>MHNDKDLSTWQTFRRLWPTIAPFKAGLIVAGIALILNAASDTFMLSLLKPLLDDGFGKTDRSVLLWMPLVVIGLMILRGITSYISSYCISWVSGKVVMTMRRRLFGHMMGMPVAFFDKQSTGTLLSRITYDSEQVASSSSGALITVVREGASIIGLFIMMFYYSWQLSIILVVLAPIVSIAIRVVSKRFRSISKNMQNTMGQVTTSAEQMLKGHKEVLIFGGQEVETKRFDKVSNKMRLQGMKMVSASSISDPIIQLIASLALAFVLYAASFPSVMDSLTAGTITVVFSSMIALMRPLKSLTNVNAQFQRGMAACQTLFAILDSEQEKDEGKRVIDRATGDLEFRNVTFTYPGREVPALRNINLKIPAGKTVALVGRSGSGKSTIASLITRFYDIDEGHILMDGHDLREYTLASLRNQVALVSQNVHLFNDTVANNIAYARTEEYSREQIEEAARMAYAMDFINKMDNGLDTIIGENGVLLSGGQRQRIAIARALLRDSPILILDEATSALDTESERAIQAALDELQKNRTSLVIAHRLSTIEQADEIVVVE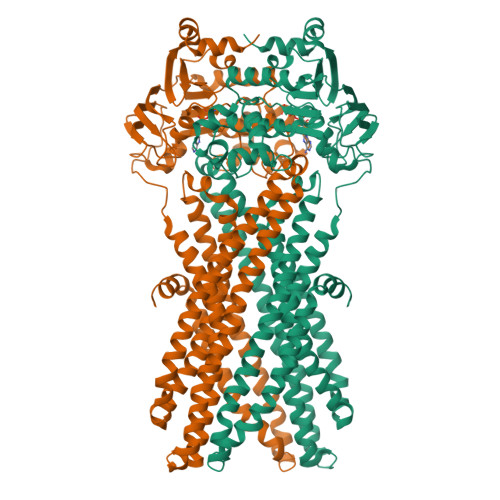DGIIVERGTHSELLAQHGVYAQLHKMQFGQ[4x]> GPLGSGKKCYKLENEKLFEEFLELCKMQTADHPEVVPFLYNRQQRAHSLFLASAEFCNILSRVLSRARSRPAKLYVYINELCTVLKAHSAKKKLN;> SENRIAKKMLLEEIKANLSSDED

Alpha-thalassemia/mental retardation syndrome X-linked protein (ATRX) is a member of the switch 2/sucrose nonfermentable 2 (SWI2/SNF2) family of chromatin-remodeling proteins. ATRX deposits histone variant H3.3 into heterochromatin loci with the cooperation of an H3.3-specific chaperone, the death-domain associated protein (DAXX). The DAXX helical bundle (DHB) domain has been shown to interact with two modules of ATRX. The DAXX-ATRX interaction is a crucial link to bridge the chaperone-activity domain of DAXX and the remodeling-activity domain of ATRX together to deposit H3.3 into heterochromatin foci.

We determined the structure of the DAXXDHB–ATRXDBM complex at a resolution of 2.2 Å using single-wavelength anomalous dispersion with selenomethionine-substituted crystals. The final refined model covered DAXX residues 57–141 and ATRX residues 1,267–1,284. DAXXDHB forms an elongated helix bundle with four antiparallel packed helices α1, α2, α4, and α5. α3 is a short helix connecting α2 and α4, and it crosses the base of the helical bundle. ATRXDBM exists as a long amphipathic helix (residues 1,269–1,283) lying along the cleft between helices α2 and α5 of DAXXDHB. ATRXDBM binding does not induce large conformational change in DAXXDHB, because the DAXXDHB structure in the complex is almost identical to the previously determined NMR structure of apo DAXXDHB, with a root-main-square deviation (rmsd) value of 1.0 Å for 83 equivalent Cα pairs. The interaction between DAXXDHB and ATRXDBM is predominantly mediated by hydrophobic contacts. Four nonpolar residues (A1272, L1276, L1277, and I1280) in the center of the ATRXDBM helix constitute a hydrophobic core that fits snugly into a shallow groove in DAXXDHB. The side chains of these residues make close contacts with a panel of hydrophobic amino acids, including V84, F87, Y124, V125, and I127 of DAXX. Complementary with the hydrophobic contacts, a series of salt bridges and hydrogen-bonding interactions further strengthened the interactions between DAXXDHB and ATRXDBM. Moreover, our structural analyses of DAXXDHB-ATRXDBM and DAXXDHB-RASSF1CDBM indicate that DAXXDHB is a general protein-interaction domain with sufficient structural plasticity to accommodate DBMs from different interaction partners.>[4x]MVQQKVEVRLKTGLQARPAALFVQE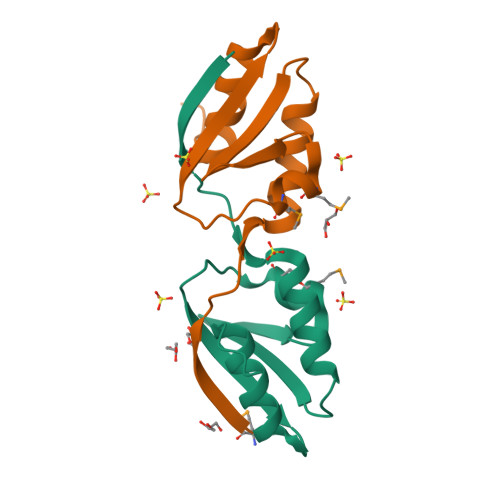ANRFTSDVFLEKDGKKVNAKSIMGLMSLAVSTGTEVTLIAQGEDEQEALEKLAAYVQEEVLQ> GSEMSVVEYEVVSKNLTSKMSHELLFSVKKRWFVKPFRHD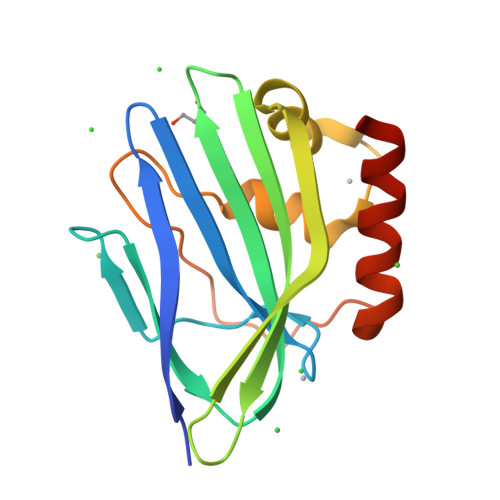RQLGKLHYKLLPGNYIKFGLYVLKNQDYARFEIAWVHVDKDGKIEERTVYSIETYWHIFIDIENDLNCPYVLAKFIEMRPEFHKTAWVEESNYSIAEDDIQMVESIKRYLERKIASD>SMAEAASEIPEKFFGKYDLDRSENFDEFLAAKGVSWFVRQMIKLAKVSKVLAKNETPGKYNMENLTSKKNTLYHGWELGKTFEAEGLDGVAHKITFSFKDGVLSEHHIRLNDPEHSAETYYYTIENDQLVMKMVNNGITCRRWFKRSTGKK[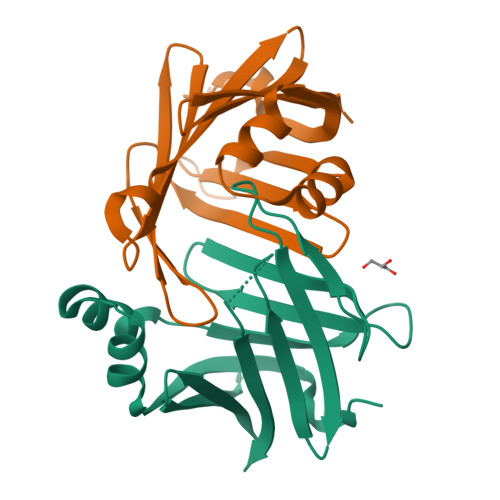2x]> GGSMNKLYIGNLSENAAPSDLESIFKDAKIPVSGPFLVKTGYAFVDCPDESWALKAIEALSGKIELHGKPIEVEHSVPKRQ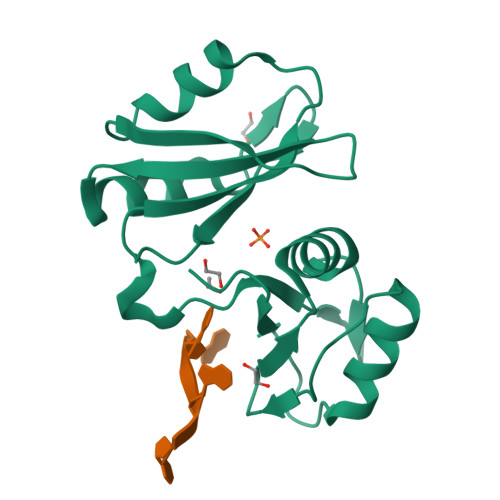RIRKLQIRNIPPHLQWEVLDSLLVQYGVVESCEQVNTDSETAVVNVTYSSKDQARQALDKLNGFQLENFTLKVAYIPDEMAAQHHHHHH>[2x]HHHGQPPSGYGVLLATHDDDTVDVFTSGRKMRLTCSPNIDAASLKKGQTVRLNEALTVVEAGTFEAVGEISTLREILADGHRALVVGHADEERVVWLADPLIGGGPRKLRPGDSLLVDTKAGYAFERIP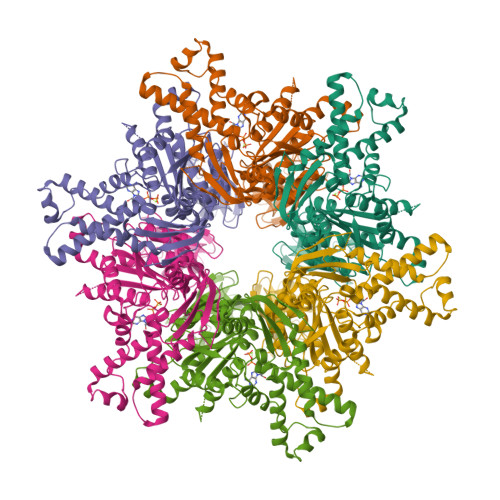KAEVEDLVLEEVPDVSYADIGGLSRQIEQIRDAVELPFLHKELYREYSLRPPKGVLLYGPPGCGKTLIAKAVANSLAKKMAEVRGDDAHEAKSYFLNIKGPELLNKFVGETERHIRLIFQRAREKASEGTPVIVFFDEMDSIFRTRGTGVSSDVETTVVPQLLSEIDGVEGLENVIVIGASNREDMIDPAILRPGRLDVKIKIERPDAEAAQDIYSKYLTEFLPVHADDLAEFDGDRSACIKAMIEKVVDRMYAEIDDNRFLEVTYANGDKEVMYFKDFNSGAMIQNVVDRAKKNAIKSVLETGQPGLRIQHLLDSIVDEFAENEDLPNTTNPDDWARISGKKGERIVYIRTLVTGKSSSASRAIDTE> SGNFCPLCDKCYDDDDYESKMMQ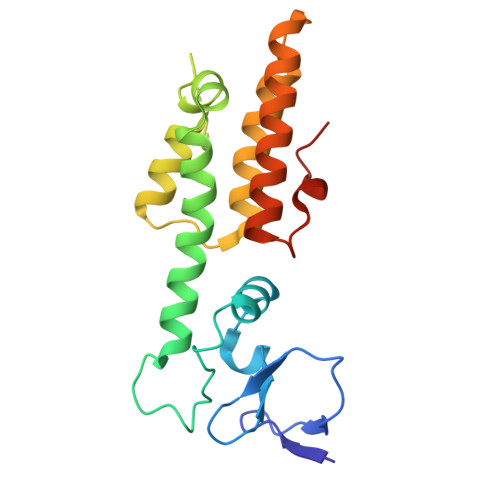CGKCDRWVHSKCENLSDEMYEILSNLPESVAYTCVNCTERHPAEWRLALEKELQISLKQVLTALLNSRTTSHLLRYRQQQPLDLEGVKRKMDQGNYTSVLEFSDDIVKIIQAAINSDGGQPEIKKANSMVKSFFIRQMERVFPWFSVKKSRFWEPNKVSS>GMSKSENAGQRPHVAVFPCAGMGHLLPYLRLAAMLHSRGCAVSVISAHPTISDAESRSLSSFFSLYPQIRSLEIQLLPLKRNPRFTNDDPFFIQRESIGNSIHLLRPLLASLSPPLSAIFVDFPVLTEFSPIAADFSLPTYTLIVTSARFFSLMAHLPRLLEQEDDISKKSEVCVPHLDPIQVSSIPPQMLDRRHFFVETITSNVASLSYLKGVLINTFTWLEPEAVEALKRNGVDHILPIGPLEAIKAEESDMDLPWLEEQAPKSVLFISFGSRGAHTKEQLREFAAALEKSGWRFLWVLKSGKVDREDKEETEDILGSSFLERTKNRGVVIKGWADQERILAHSAIGGFVSHCGWNSVVEAAKLGVPVLAWPPHGDQRVNAEVVEKVGLGLWVRGWGWAGERLIGRDEIAEKLIELRNDERLRERVKEVREKAREERESGGISETLIRD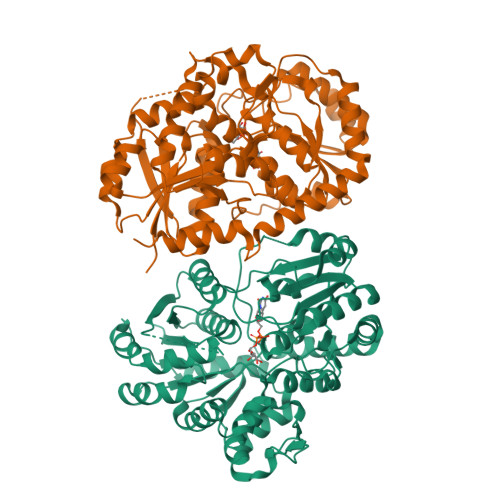LIHSLKIK[2x]Here, we report the crystal structure of the Lit enzyme from Bacillus cereus and describe its mechanism of action. Lit consists of four transmembrane helices with an extracellular cap. Conserved residues map to the cap-membrane interface. They include two catalytic histidines that function to effect unimolecular transacylation. The reaction involves acyl transfer from the sn-2 position of the glyceryl moiety to the amino group on the N-terminal cysteine of the substrate via an 8-membered ring intermediate.

Two structures were solved; one at 2.27 Å, the other at 1.95 Å. Here, we focus on molecule B (MolB) in the 1.95 Å structure, which has the better quality electron density. The protein assumes the shape of a truncated cone that spans the membrane with four transmembrane helices (M1–M4). Notably, two structured monoolein molecules that derive from the crystallisation process reside with their glyceryl head groups coordinated with the two conserved histidines. The sn-2 hydroxyl of MO1 coordinates with His85. The sn-3 hydroxyl of MO2 coordinates with His85 and His153. In MolB of the asymmetric unit, the chains run parallel to one another below the apolar surface of amphiphilic H4. In the apo form of Lit, M3 is bent midway along its length between Pro134 and Pro140.

>MHHHHHHSSGRENLYFQGHMDRLITLVVSYSIAFSIFALATMAVVYGKWLYYFEIDFLNIPDLADMTKDEIKRNYDVLITYLSPFYDGALHLPTLDMSTNGRIHFVDVKNILVKIQYVMYATIMIAVIGGIYLLKKKNEKFLLHGSILTIIFPIALMLPIAINFEKSFVLFHKLLFSNDYWVFDPEKDPIILMLPEEFFMHAACAILLFILGGSILCYSLYRYLVKKKRMSQKKFSA[2x]> MSLEVKVGLAPMAGYTDSAFRTLAFEWGADFAFSEMVSAKGFLMNSQKTEELLPQPHERNVAVQIFGSEPNELSEAARILSEKYKWIDLNAGCPVRKVVKEGAGGALLKDLRHFRYIVRELRKSVSGKFSVKTRLGWEKNEVEEIYRILVEEGVDEVFIHTRTVVQSFTGRAEWKALSVLEKRIPTFVSGDIFTPEDAKRALEESGCDGLLVARGAIGRPWIFKQIKDFLRSGKYSEPSREEILRTFER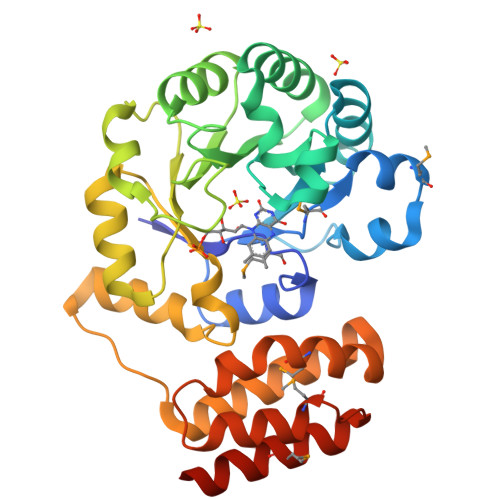HLELLIKTKGERKAVVEMRKFLAGYTKDLKGARRFREKVMKIEEVQILKEMFYNFIKEVEGGSHHHHHH(2E)-3-(3-chloro-5-{2-[2-(2,4-dioxo-3,4-dihydropyrimidin-1(2H)-yl)ethoxy]phenoxy}phenyl)prop-2-enenitrile 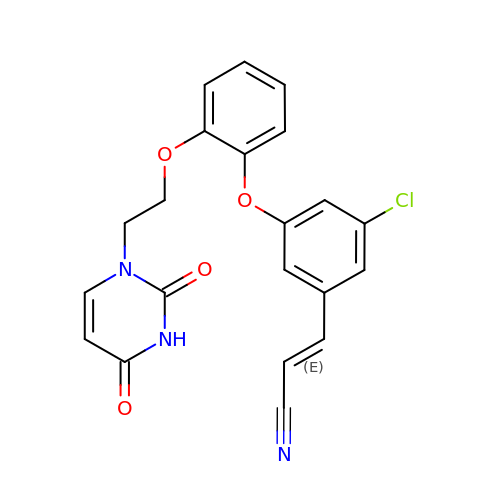| C21 H16 Cl N3 O4 | QQWLDKMLZHRQRI-ONEGZZNKSA-N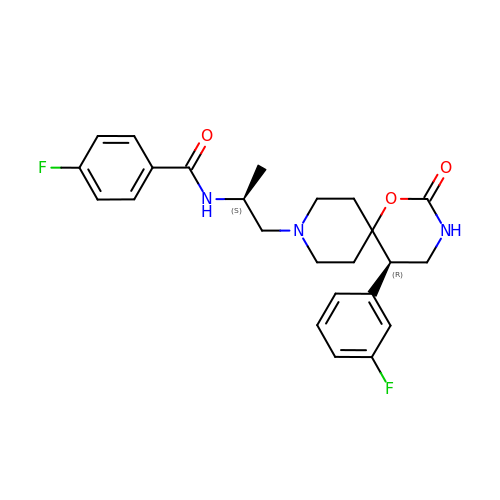4-fluoro-N-{(2S)-1-[(5R)-5-(3-fluorophenyl)-2-oxo-1-oxa-3,9-diazaspiro[5.5]undecan-9-yl]propan-2-yl}benzamide | C24 H27 F2 N3 O3 | QLCFHHJOCOKGIV-KKSFZXQISA-N> MSGSLREEIRKLAEQLSEKYKDEEIRELAREAAELAEESDDPEVLELAYEALKKGLELEDEEKVKLILLAAVLAARVARGEVPEEKLEIALKALELAEASEDERIIRGALRAALAAARTDDPLALEVVLEALERAQASEDERLIRAILAAAYAFALLAVAGASAERLKEAEAIVKELIAAAEKGASPQELVLLVIEMMVKGMGVTMETHRSGNEVKVVIKGL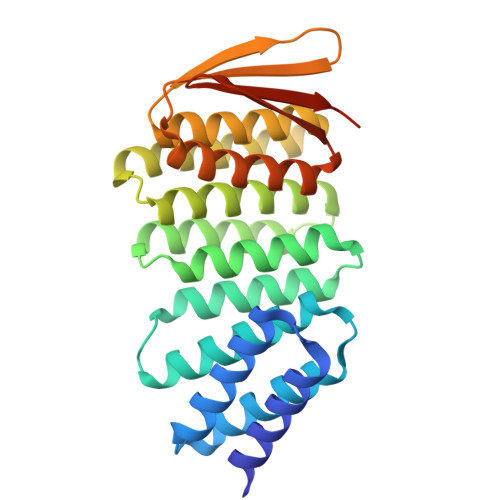HESQQEVLLEAVLFAAELMGVRVRIRFKGDTVTIVVREGSGSHHWGSTHHHHHH> MGSSHHHHHHSQDPNSMTTLTRQDLNFGQVVADVLCEFLEVAVHLILYVREVYPVGIFQKRKKYNVPVQMSCHPELNQYIQDTLHCVKPLLEKNDVEKVVVVILDKEHRPVEKFVFEITQPPLLSISSDSLLSHVEQLLAAFILKISVCDAVLDHNPPGCTFTVLVHTREAATRNMEKIQVIKDFPWILADEQDVHMHDPRLIPLKTMTSDILKMQLYVEERAHKGS;> MRGSHHHHHHGSGLSSLQSDPAGCVRPPAPNL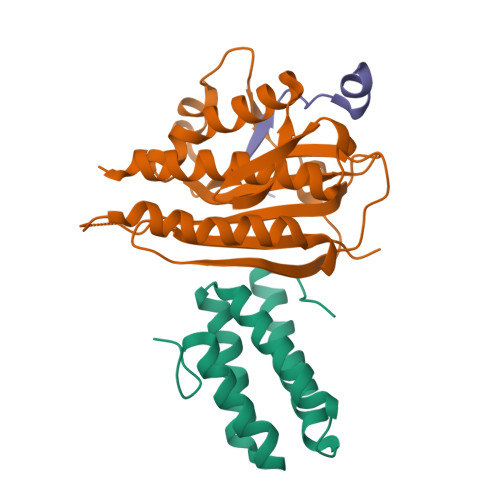AGAVEFNDVKTLLREWITTISDPMEEDILQVVKYCTDLIEEKDLEKLDLVIKYMKRLMQQSVESVWNMAFDFILDNVQVVLQQTYGSTLKVT;> MLTPTPDSSPRSTSSPSQSKNGSFTPRTANILKPLMSPPSREEIMATLLDHD> CIEEGQYCFAD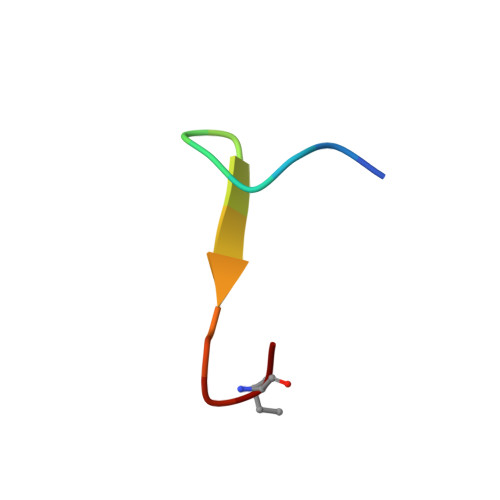PYLC> MKVNMEYTKEKKVGEGTYAVVYLGCQHSTGRKIAIKEIKTSEFKDGLDMSAIREVKYLQEMQH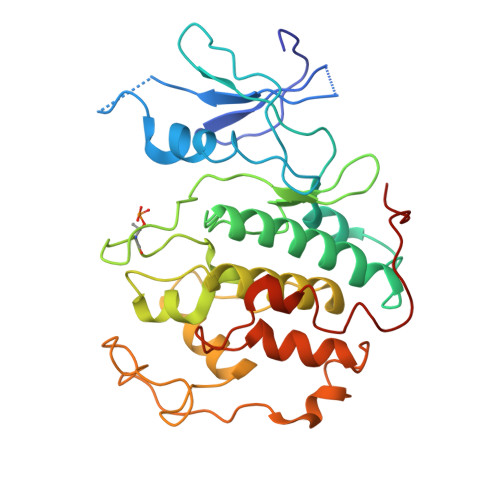PNVIELIDIFMAYDNLNLVLEFLPTDLEVVIKDKSILFTPADIKAWMLMTLRGVYHCHRNFILHRDLKPNNLLFSPDGQIKVADFGLARAIPAPHEILTSNVVTRWYRAPELLFGAKHYTSAIDIWSVGVIFAELMLRIPYLPGQNDVDQMEVTFRALGTPTDRDWPEVSSFMTYNKLQIYPPPSRDELRKRFIAASEYALDFMCGMLTMNPQKRWTAVQCLESDYFKELPPPSDPSSIKIRN> GSGSDQSPKPLATRDEKITYLRKIIGDKGSDAWDVAWQEGVTPWDQGKIQPPLRDFIESNDGKALVNKKSDNARVLVPGCGKGYDAAYFASLGYETLGADLSSTAIEKAKEFWAESPELKSGKLSFQTLDFFKFEVPEAKYDLVYDYTFFCALPPDLRAPWGARMRELVRPGGTLITLVYPIDGARSGGP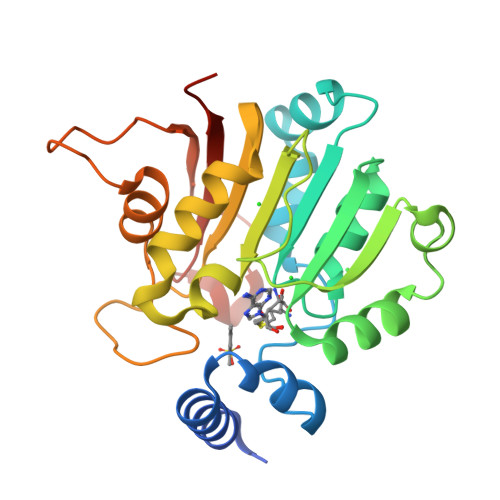PYSIDVQKVTDALQGSEEGSAEPGKYWTKVLDIVPQTSSPDHVGRERLVVWERINKPLQDKL> XGPPGPKGPKGD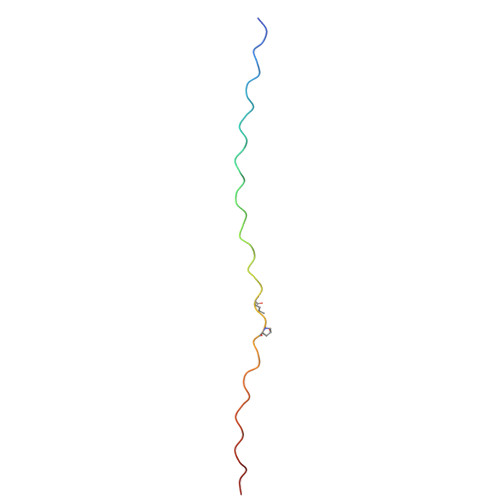PGDPGPPGARGQAGVLGFPGPPGPKGPKGDPGDP>SAPVSIWSRVVQFGTGWGFWVSGHVFITAKHVAPPKGTEIFGRKPGDFTVTSSGDFLKYYFTSAVRPDIPAMVLENGCQEGVVASVLVKRASGEMLALAVRMGSQAAIKIGSAVVHGQTGMLLTGSNAKAQDLGTIPGDAGCPYVYKKGNTWVVIGVHVAATRSGNTVIAATHGEPTLEALEFQG[4x];> LEFQG

Whereas ORF2, ORF3 and ORF4 each encode single proteins, ORF1 codes for a large polyprotein (∼190 kDa) that is processed by the virally-encoded protease at five specific sites to release the six ‘mature’ non-structural proteins (NS1/2–NS7)—and an array of functional precursors—that are required for virus replication. The viral NS6 protease present within the C-terminal half of the polyprotein performs all the processing, including its own autocatalytic release from the precursor (Liu, Clarke & Lambden, 1996; Belliot et al., 2003; Sosnovtsev et al., 2006; Scheffler et al., 2007). Norovirus NS6 is a cysteine protease with a chymotrypsin-like fold: two β-barrel domains separated by a cleft that contains a Cys-His-Asp/Glu catalytic triad similar in arrangement to the Ser-His-Asp triad characteristic of serine proteases. To this end we extended an inactive MNV NS6 construct (which incorporates a C139A mutation to knock out the active site nucleophile) by adding residues from NS7, which is immediately downstream in the polyprotein.

We made three constructs, NS6 1′, NS6 2′ and NS6 4′, which were extended by 1, 2 and 4 residues respectively, generating proteases that contain substrates that correspond to P4–P1′, P4-P2′ and P4-P4′ of the NS6–NS7 cleavage junction. MNV NS6 1′ crystallised in space group C2 with four molecules in the asymmetric unit. This structure is notable for the fact that, in contrast to the other three structures reported here and the structures previously reported for Norwalk virus NS6 protease (Zeitler, Estes & Prasad, 2006; Muhaxhiri et al., 2013), the electron density map was of sufficient quality in all four molecules of the asymmetric unit to permit the incorporation of the loop between the β-strands cII and dII. Superposition of the four copies of NS6 1′ indicates some structural variation in this loop—the Cα positions vary by 1–2 Å—consistent with the notion that it is rather flexible. In three of the molecules in the asymmetric unit the C-terminus is disordered beyond residue 173 (chains A and D) or residue 174 (chain C). Although the full C-termini of chains A, C and D of the NS6 1′ could not be modelled, the electron density map revealed additional features that could be built as short stretches of polypeptide. These correspond to portions of the missing C-termini but, because of discontinuities in the electron density, it is not possible to unambiguously ascribe which monomer they belong to. In contrast to chains A, C and D, the electron density for the B chain in the asymmetric unit was sufficiently clear to permit inclusion of all 183 residues of NS6 and the extra first residue of NS7 (here labelled Gly 184) in the refined model. The C-terminus of Chain B of NS6 1′ beyond Gly 173 extends to make contacts with chain B from an adjacent asymmetric unit to which it is related by a two-fold symmetry axis.>[2x]MIDLRSDTVTRPSRAMLEAMMAAPVGD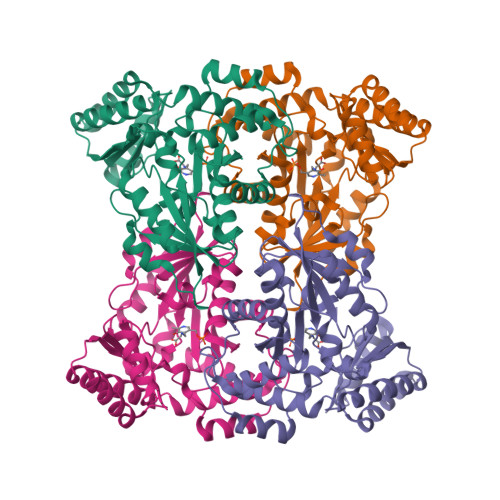DVYGDDPTVNALQDYAAELSGKEAAIFLPTGTQANLVALLSHCERGEEYIVGQAAHNYLFEAGGAAVLGSIQPQPIDAAADGTLPLDKVAMKIKPDDIHFARTKLLSLENTHNGKVLPREYLKEAWEFTRERNLALHVDGARIFNAVVAYGCELKEITQYCDSFTICLSKGLGTPVGSLLVGNRDYIKRAIRWRKMTGGGMRQSGILAAAGIYALKNNVARLQEDHDNAAWMAEQLREAGADVMRQDTNMLFVRVGEENAAALGEYMKARNVLINASPIVRLVTHLDVSREQLAEVAAHWRAFLAR>[4x]MKLEHKNIFITGSSRGIGLAIAHKFAQAGANIVLNSRGAISEELLAEFSNYGIKVVPISGDVSDFADAKRMIDQAIAELGSVDVLVNNAGITQDTLMLKMTEADFEKVLKVNLTGAFNMTQSVLKPMMKAREGAIINMSSVVGLMGNIGQANYAASKAGLIGFTKSVAREVASRNIRVNVIAPGMIESDMTAILSDKIKEATLAQIPMKEFGQAEQVADLTVFLAGQDYLTGQVIAIDGGLSM

One critical component of FAS II system is 3-oxoacyl-[acyl-carrier-protein] reductase (FabG), which plays a vital role in the elongation process necessary for the production of both saturated and unsaturated fatty acids, utilizing NADPH to catalyze the initial reduction step, facilitating the conversion of 3-oxoacyl-ACP to 3-hydroxyacyl-ACP intermediates. Recent research has identified fabG of S. pneumoniae as an essential gene through CRISPRi assay, indicating that SpFabG may be a promising target for the development of anti-S. pneumoniae agents. The strains carrying plasmids producing either functional FabGs or the yeast OAR1 exhibited the same growth as the wild-type strains. These demonstrated that SpFabG has the capability to complement both E. coli and yeast in vivo, thereby functioning as 3-oxoacyl-[acyl-carrier-protein] reductase FabG. When SpFabG amino acid sequence was investigated through multiple sequence alignment, there is a conserved NADPH binding site along with the Ser-Tyr-Lys active triad responsible for substrate catalyzation.

We have determined the crystal structure of SpFabG at 2 Å resolution using AlphaFold predicted monomer as template for molecular replacement, shows casing its similarity to the overall fold of the E. coli FabG. In the asymmetric unit of the crystal form, there is a single tetramer. Despite the slight differences in the flexible region among the monomers, this analysis primarily focuses on the structure of the most stable monomer, chain A. Overall, the protein conforms to a Rossmann fold, with its core comprising a twisted, parallel β sheet consisting of seven β strands flanked on both sides by a total of eight α helices. The active-site residues (Ser140, Tyr153, and Lys157) are clustered near the loop connecting β5 and α5. The conformation observed in the crystal structure is considered to be inactive conformation, with the Ser140-containing β5-α5 loop occupying the pocket where the nicotinamide part of the ligand should be. In three out of the four monomers in the asymmetric unit, this loop is stabilized by a crystal contact, and the electron density clearly reveals both the conformation of the loop and the active triad. Phe223 in the α8 interface plays a crucial role by facilitating a π- π stacking and attracting the relevant side chains towards each other, and Ala236 in the β7 interface interacts with Gln233 in β7′ by forming a hydrogen bond. It is noteworthy that the hydrophobic side chain of Tyr229 inserts into a hydrophobic pocket on the neighboring side, resembling a key inserting a lock. The interface B, locates between helices α4, α5 and their respective counterparts in the neighboring monomer (α4′, α5′), constitutes a four-helix bundle.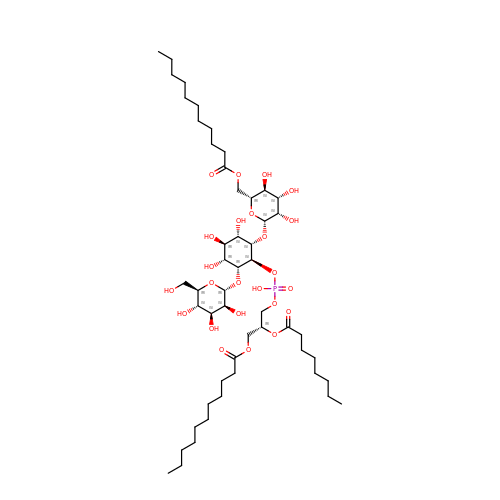(2R)-3-{[(R)-hydroxy({(1S,2R,3R,4R,5S,6S)-3,4,5-trihydroxy-2-(alpha-D-mannopyranosyloxy)-6-[(6-O-undecanoyl-beta-D-mannopyranosyl)oxy]cyclohexyl}oxy)phosphoryl]oxy}-2-(octanoyloxy)propyl undecanoate | C51 H93 O24 P | QGXVEMBXLAEQBM-PUGXMYIYSA-N> AAQPAEECMHASGENYDGKISKTMSGLECQAWDSQSPHAHGYIPSKFPNKNLKKNYCRNPDRELRPWCFTTD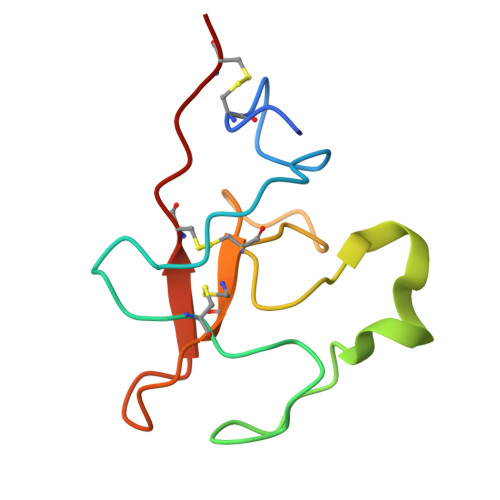PNKRWELCDIPRCTT>MDTNPCEKHSCIAVIDAGSTGSRLHIYSYDTDDTNTPIHIEEIWNKKIKPGFASIQPNSVTIDAYLTMLLADAPIHNIPVYFYATAGMRLLPQSQQKKYYDELDYWFRQQSQWQLVEAKTITGNDEALFDWLAVNYKLDTLKSVQNKSVGVMDMGGASVQIVFPMPKNAEISKHNQVELNIYGQNINLYVHSFLGLGQTEMSHQFLNSPSCFANDYPLPDGESGQGNAPSCKEEVTSLMNSVHKVNQQIQPLLALNP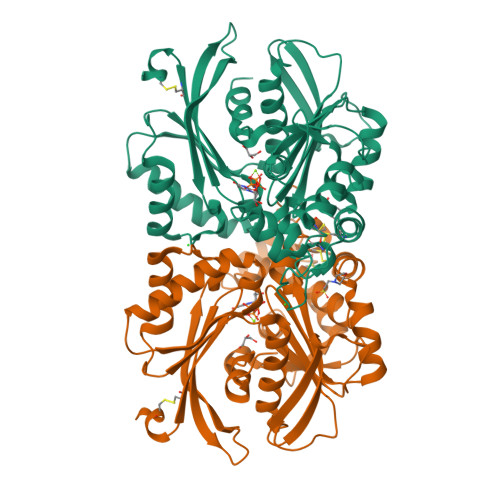VNEWYSIGGISYLASSQLFHFENSELTNQSLLQQGDNQICHQQWDILNGQYPDDEYLYQYCLLSSYYYALMVDGYGINPNQTIHYIPPEQNLDWTIGVVLHRALEHHHHHH[2x]The present work focuses on the group A endonuclease (DNase) colicin, ColE9, a member of the E group of colicins (ColE2‐E9), all of which use the same import machinery but target different nucleic acids in the cytoplasm (DNA, rRNA or tRNAs). At its N‐terminus is an 83 amino acid intrinsically unstructured translocation domain (IUTD) that houses three protein‐protein interaction epitopes (Housden et al, 2010); a 16‐residue TolB‐binding epitope (TBE) associates with the periplasmic protein TolB which is flanked by two OmpF‐binding sites (OBS1 and OBS2). Escherichia coli porins OmpF and OmpC are abundant trimeric β‐barrel outer membrane proteins with narrow channels running through them that taper to an eyelet, 7–8 Å at the narrowest point. Tol‐dependent colicins assemble a translocon at the cell surface that involves its periplasmic target along with the OM receptor and translocator which together establish the import pathway of the toxin.

Single particle analysis revealed the presence of two populations of ColE9 translocon complexes, one where the translocon was intact and a second class where BtuB was absent, which we refer to as the partial translocon. The absence of BtuB in the partial translocon, most likely due to receptor dissociation during its deposition on grids, resulted in an improvement in map resolution, which varies from 3.7 to 6 Å (FSC). The partial translocon is comprised of OmpF, the IUTD and T‐domain of ColE9 and TolB. The partial translocon structure of ColE9 shows how the IUTD (residues 3–67) navigates through the lumen of one OmpF subunit in order to thread back up into a neighbouring subunit. The end result is that each OBS is lodged within an individual subunit of OmpF: OBS1 (residues 2–18) is bound to subunit 1 while OBS2 (residues 54–63) is bound to subunit 2, leaving subunit 3 free of colicin. By contrast, OBS2 spans the eyelet of OmpF subunit 2 via a kink created at Gly61, which is enforced by the hydrogen bonding of neighbouring residues, Ser60 and Arg62. In addition to these interactions, networks of hydrogen bonds lock OBS1 and OBS2 of ColE9 into defined conformations within their respective OmpF subunits. Importantly, rotation of the ColE9 T‐domain from the full to the partial translocon repositions ColE9 from a central position above the OmpF trimer to become localised above subunit 2 within which OBS2 is bound. The position of TolB is rotated by ˜50° between the two structures and in the partial translocon is located closer to OmpF through a ˜8 Å upward movement along the axis of rotation. The positioning of TolB closer to OmpF in the partial translocon structure is stabilised by additional interactions between the periplasmic region of OmpF subunit 1 and the IUTD sequence immediately preceding the TBE.

>[3x]AEIYNKDGNKVDLYGKAVGLHYFSKGNGENSYGGNGDMTYARLGFKGETQINSDLTGYGQWEYNFQGNNSEGADAQTGNKTRLAFAGLKYADVGSFDYGRNYGVVYDALGYTDMLPEFGGDTAYSDDFFVGRVGGVATYRNSNFFGLVDGLNFAVQYLGKNERDTARRSNGDGVGGSISYEYEGFGIVGAYGAADRTNLQEAQPLGNGKKAEQWATGLKYDANNIYLAANYGETRNATPITNKFTNTSGFANKTQDVLLVAQYQFDFGLRPSIAYTKSKAKDVEGIGDVDLVNYFEVGATYYFNKNMSTYVDYIINQIDSDNKLGVGSDDTVAVGIVYQF;> MSGGDGRGHNTGAHSTSGNINGGPTGIGVSGGCSDGSGWSSENNPWGGGSGSGIHWGGGSGRGNGGGNGNSGGGSGTGGNLSAVAAPVAFGFPALSTPGAGGLAVSISASELSAAIAGIIAKLKKVNLKFTPFGVVLSSLIPSEIAKDDPNMMSKIVTSLPADDITESPVSSLPLDKATVNVNVRVVDDVKDERQNISVVSGVPMSVPVVDAKPTERPGVFTASIPGAPVLNISVNDSTPAVQTLSPGVTNNTDKDVRPAGFTQGGNTRDAVIRFPKDSGHNAVYVSVSDVLSPDQVKQRQDEENRRQQEWDAT;> MKQALRVAFGFLILWASVLHAEVRIVIDSGVDSGRPIGVVPFQWAGPGAAPEDIGGIVAADLRNSGKFNPLDRARLPQQPGSAQEVQPAAWSALGIDAVVVGQVTPNPDGSYNVAYQLVDTGGAPGTVLAQNSYKVNKQWLRYAGHTASDEVFEKLTGIKGAFRTRIAYVVQTNGGQFPYELRVSDYDGYNQFVVHRSPQCLMSPAWSPDGSKLAYVTFESGRSALVIQTLANGAVRQVASFPRHNGAPAFSPDGSKLAFALSKTGSLNLYVMDLASGQIRQVTDGRSNNTEPTWFPDSQNLAFTSDQAGRPQVYKVNINGGAPQRITWEGSQNQDADVSSDGKFMVMVSSNGGQQHIAKQDLATGGVQVLSSTFLDETPSLAPNGTMVIYSSSQGMGSVLNLVSTDGRFKARLPATDGQVKFPAWSPYL> MLKRCYLLILLMFVLASCAHHKPQTPPAEVKKQGTSSTRQFRQVSSFNQIVVQGRLNVNLHTGYNKPEVMLRGDPRDLVQVRTIVKQNTLYVSLGQGYPDYGAVTVDIKTKFLNRFRYEGAGVVTGNNLRTSYLDLYLANEGTTRLAGNIGLQKLEAVGNGVTQINGVSSRNLQIVLKGDPKVLIS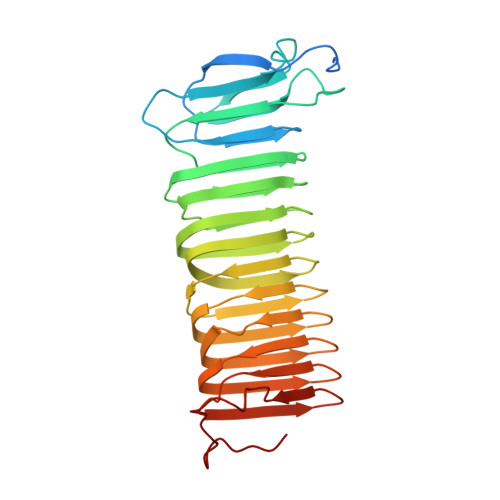GFVNLRQLDMYGKGTLSLYWIKSDTLTIRAKKAAKIQLAGIVNRLDVELWDFAQFKGKYLRAQRSFVKTHDKSVAEISAVNHQSSLATDASDIYYYNLSKTRADFMAFNGSVLDMREWGQSDLKDFDRYNKQFP>FRRQLKKLDEDSLTKQPEEVFDVLEKLGEGSYGSVYKAIHKETGQIVAIRQVPVESDLQEIIKEISIMQQCDSPHVVKYYGSYFKNTDLWIVMEYCGAGSVSDIIRLRNKTLTEDEIATILQSTLKGLEYLHFMRKIHRDIKAGNILLNTEGHAKLADFGVAGQLTDTMAKRNTVIGTPFWMAPEVIQEIGYNCVADIWSLGITAIEMAEGKPPYADIHPMRAIFMIPTNPPPTFRKPELWSDNFTDFVKQCLVKSPEQRATATQLLQHPFVRSAKGVSILRDLINEAMDVKLKRQESQQRE[2x];>[2x]AQGLAMYLQENGIDCPKCKFSYALARGGCMHFHCTQCRHQFCSGCYNAFYAKNKCPEPNCRVKKSLHGHHPRDCLFYLRDWTALRLQKLLQDNNVMFNTEPPAGARAVPGGGCRVIEQKEVPNGLRDEACGKETPAGYAGLCQAHYKEYLVSLINAHSLDPATLYEVEELETATERYLHVRPQPLAGEDPPAYQARLLQKLTEEVPLGQSIPRRR

HOIP, an RBR-type E3 ligase and the catalytic subunit of the linear ubiquitin chain assembly complex (LUBAC), plays crucial roles in various cellular processes, including the NF-κB signaling pathway. Particularly, STK4 can directly phosphorylate HOIP and inhibit its E3 activity, thereby attenuating the LUBAC-mediated activation of the NF-κB signaling pathway. As a serine/threonine kinase, STK4 specifically recognizes and phosphorylates dozens of protein substrates, including Mob1A/Mob1B, Lats1/Lats2, histone H2B, FOXO3 and HOIP, thereby regulating their relevant cellular functions. In this study, using biochemical, mass spectrometry and structural approaches, we systemically characterize the association of STK4 with HOIP, and unveil that STK4 can directly bind to the RING2-LDD module of HOIP through its kinase domain.

Therefore, we only mixed HOIP (residues 854–1072) and STK4 KD in a 1:1 molar ratio, and conducted relevant crystal screening using this protein mixture. Fortunately, this approach successfully yielded good crystals that diffracted to a 2.8 Å resolution. In the final crystal structure, each asymmetric unit contains one STK4 KD dimer and two HOIP RING2-LDD molecules, forming a symmetrical butterfly-like hetero-tetramer. Intriguingly, within the HOIP RING2-LDD/STK4 KD complex, the two STK4 KD monomers, each adopting a canonical KD-fold consisting of an N-lobe and C-lobe (but lacking an ATP molecule due to the K59R mutation), directly pack with each other to form a symmetrical dimer through their N-lobes. In parallel, the RING2 and LDD modules of each HOIP RING2-LDD pack together to form a unique architecture that is mainly composed of six α-helices and six β-strands, and coordinates four zinc ions. Specifically, through its RING2 region together with the β5 and β6 strands within the LDD domain, HOIP RING2-LDD specifically binds to the C-lobe of STK4 KD. Detailed structure analyses uncovered that the binding interface between HOIP RING2-LDD and STK4 KD is primarily formed by residues from the α7-helix of STK4 KD, which accommodates HOIP residues located in the α1-helix and β2-strand of HOIP RING2, as well as the β5- and β6-strands of HOIP LDD through both hydrophobic and polar interactions. Specifically, the side chains of S877, Q974 and D983 of HOIP form hydrogen bonds with the side chains of STK4 T238 and R231, and the backbone amide group of STK4 H228, respectively. Moreover, an Arg-Glu pair (Arg231STK4-Glu983HOIP) of salt bridge further strengthens the HOIP RING2-LDD/STK4 KD interaction.> CSCSPVHPQQAFCNADVVIRAKAVSEKEVDSGNDIYGNPIKRIQYEIKQIKMFKGPEKDIEFIYTAPSSAVCGVSLDVGGKKEYLIAGKAEGDGKMHITLCDFIVPWDTL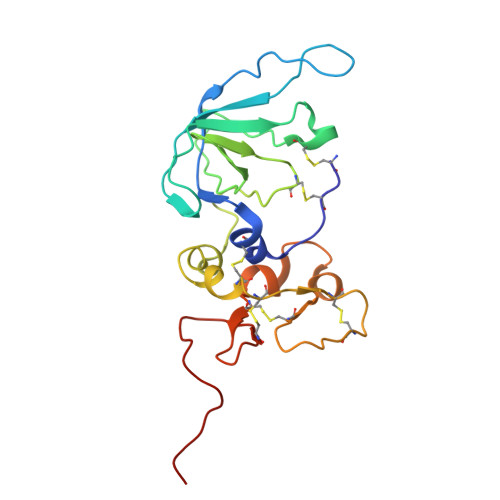STTQKKSLNHRYQMGCECKITRCPMIPCYISSPDECLWMDWVTEKNINGHQAKFFACIKRSDGSCAWYRGAAPPKQEFLDIEDP2-amino-8-cyclopentyl-4-methyl-6-(1H-pyrazol-4-yl)pyrido[2,3-d]pyrimidin-7(8H)-one 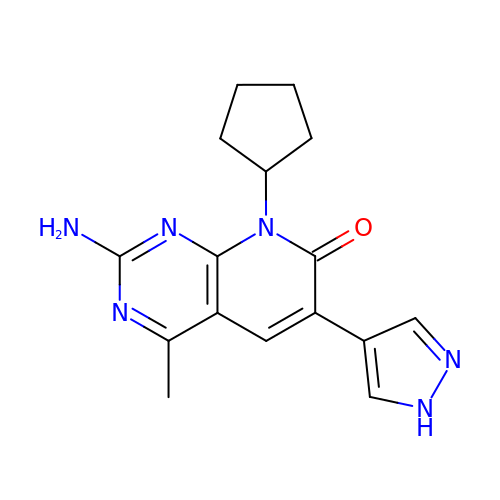| C16 H18 N6 O | VMGMCPMGGFUNMP-UHFFFAOYSA-N> MSRNYEKLSIEEFGAHLLGTVDLDPIYLALRRMELPEAQLNRWLLAYWCLYNGGEASYLSEFEGREFFEMLNHAAENVREAPIGGRWPRGAERRHWRGAQATSSVEYLIDRYDDRPEDMAAYCAGQGGTFLEVTKRVQEHRLFGPWIGFKVADMVDRVLGKPVSFDNAAVFMFKDPYKAACIQYEVNPNIPDHVLADGSVAPRNRELVTPETVHHVAQHLIEHFKGFQAPPLGDRPV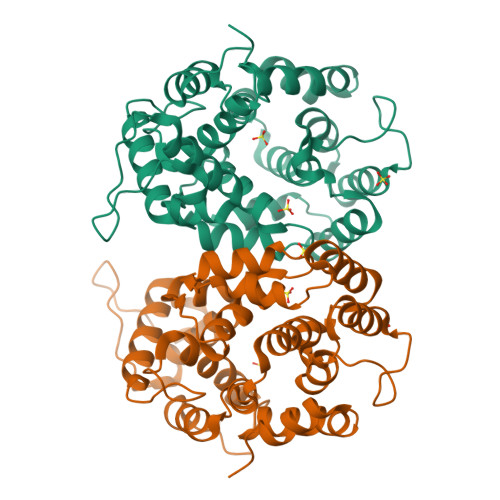NIQEVETILCKWKSHQNGHYPLFKDIVEIREAALPWAKVSKTAQAFFEAMPEVTQ>[2x]MPNSEPASLLELFNSIATQGELVRSLKAGNASKDEIDSAVKMLVSLKMSYKAAAGEDYKADCPPGNPAPTSNHGPDATEAEEDFVDPWTVQTSSAKGIDYDKLIVRFGSSKIDKE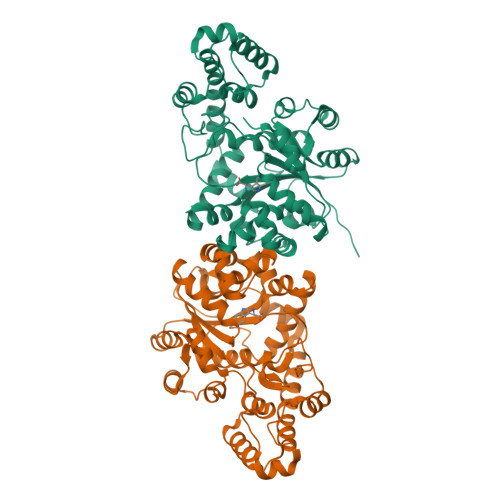LINRIERATGQRPHHFLRRGIFFSHRDMNQVLDAYENKKPFYLYTGRGPSSEAMHVGHLIPFIFTKWLQDVFNVPLVIQMTDDEKYLWKDLTLDQAYSYAVENAKDIIACGFDINKTFIFSDLDYMGMSSGFYKNVVKIQKHVTFNQVKGIFGFTDSDCIGKISFPAIQAAPSFSNSFPQIFRDRTDIQCLIPCAIDQDPYFRMTRDVAPRIGYPKPALLHSTFFPALQGAQTKMSASDPNSSIFLTDTAKQIKTKVNKHAFSGGRDTIEEHRQFGGNCDVDVSFMYLTFFLEDDDKLEQIRKDYTSGAMLTGELKKALIEVLQPLIAEHQARRKEVTDEIVKEFMTPRKLSFDFQHHHHHH Bacteriophage Casadabanvirus JBD30, from the order Caudoviricetes, is a temperate phage that infects the bacterium Pseudomonas aeruginosa. The virion of bacteriophage JBD30 is composed of an icosahedral capsid, long flexible non-contractile tail, and a baseplate. Using its baseplate, JBD30 attaches to Pseudomonas aeruginosa via the bacterial type IV pilus, whose subsequent retraction brings the phage to the bacterial cell surface.

Approximately one-half of phage JBD30 virions in our sample had capsids decorated with trimers of minor capsid proteins (gp39). Similarly to auxiliary proteins of phage λ (gpD), phage YSD1 (gp16), and phage P23-45 (gp88), the minor capsid proteins of bacteriophage JBD30 form homotrimers docked on the threefold and pseudo-threefold axes. Whereas the auxiliary proteins of phages λ, YSD1, and P23-45 form an outer chainmail net with the trimers connected to each other by their N-terminal hook extensions, the minor capsid protein trimers of JBD30 are not connected. The fold of minor capsid protein of JBD30 consists of a three-stranded antiparallel β-sheet, short β-hairpin stabilized by a disulphide bond between Cys67 and Cys72, and an α-helix. Cryo-EM density of the N-terminal region of the minor capsid protein, residues 1–52, was not resolved enough to enable determination of its structure. The interactions of the minor capsid proteins with major capsid proteins are mainly electrostatic. Negatively charged minor capsid protein residues Asp96, Ser95, and Glu91 form a pocket for Lys66 from the extended loop of the major capsid protein. Lys197 from α5 helix of the peripheral domain of the major capsid protein forms a salt bridge with the minor capsid protein residue Glu198. The major capsid protein residues Glu198, Ser194 and Thr193 interact with the minor capsid protein residue Lys100. Despite low sequence identity (13.1%), the topology of the JBD30 minor capsid protein resembles the β-tadpole fold of the T4 auxiliary protein Soc.

>MAIITPALISALKTSFQKHFQDALATAPSTYLQVATVIPSTTASNTYGWLGQFPKLREWIGQRVIKDMAAQGYQITNKLFESTVGVKRTDIEDDNLGVYGPLMQEMGRAAGAHPDELVFALLKAGNANLCYDGQNFFDTDHPVYPNVDGTGTATTVSNLFAPAADPGAAWYLLDTSRSLKPLIYQERMKPSFTSMTKEDDEQVFMADEYRYGVRSRCNVGFGFWQLAAMSTEELNQVNFEKVYDAMRNQKADGGRPLDIRPNLLVVPTTLRSKAKEVVGVQRLANGADNPNFELVQVLDTAWLN[7x];>[7x]MARQNSAAKTTAKSKTDPATEKPKDDTLPDSTDDASPTAPETPATKPDSASDEVEGVFVRATVERRCRAGFCFDKEGQGFADGVLSDEQLEALESDPLLKVERCTFSGNQEGE> MVMGIFANCIFCLKVKYLPQQQKKK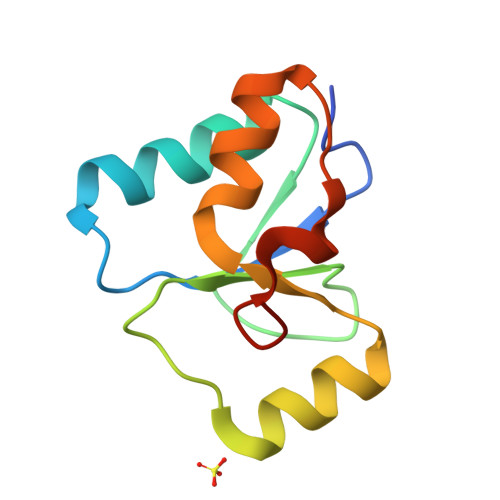LQTDIQENGGKFSFSLNPQCTHIILDNADVLSQYQLNSIQKNHVHIANPDFIWKSIREKRLLDVKNYDPYKPLDI(1R,4R,5R)-3-(tert-butylcarbamoyl)-1,4,5-trihydroxycyclohex-2-ene-1-carboxylic acid | C12 H19 N O6 | 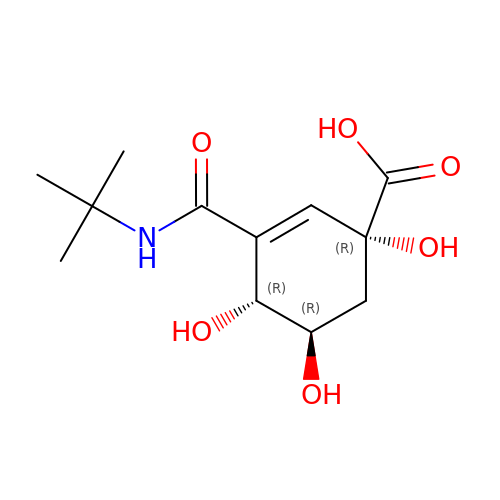BDNCEUNKGWSSTP-RWYTXXIDSA-N>[6x]MTSAEMTSPNNNSEHQAIAKMRTMIEGFDDISHGGLPIGRSTLVSGTSGTGKTLFSIQFLYNGIIEFDEPGVFVTFEETPQDIIKNARSFGWDLAKLVDEGKLFILDASPDPEGQEVVGGFDLSALIERINYAIQKYRARRVSIDSVTSVFQQYDAPSVVRRELFRLVARLKQIGATTVMTTERIEEYGPIARYGVEEFVSDNVVILRNVLEG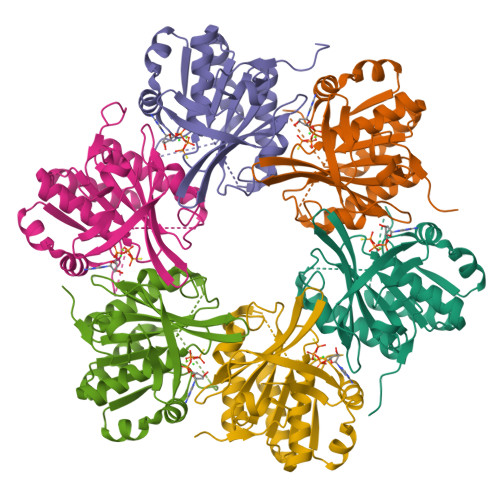ERRRRTLEILKLRGTSHMKGEYPFTITDHGINIFPLGAMR> MDVDLFKLSLDDTSSVKGSLLDTRFAQVRVVIPKAMAGGNELLNSNLYDILVVDNNFRAAAALAHTHIIEGQIKCVCTINLPENTGCCLALCVNSSNRGQFSTDIYTIGSQDRMLWNPACSKNSTFTFNPNPCGTGWSLEFLRRTKFHISVVCVSGWSAQPQTDLVMTMDFFVANVPCVPRIYNLGSPGQTLWLNRWMGKLSFGQGVSNDIKSMPLAIGGGAGAKDSILMNMTNAYLSLWRY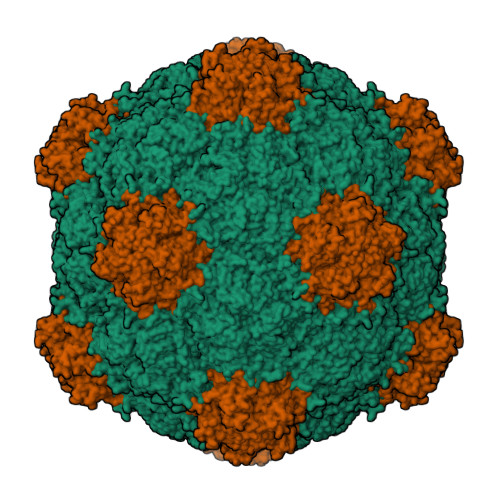FHGDLVFEVNKMSSPYIKSTVTFFIGFGGVSFQPELEDFPNKLVQFSEVQEKIELKFTRAEFLTAWSTQVDPAAQLANDGCPYLYAMVHDSTASTIVGDFNLGVTLTRIENFAGIGCNPGIQGARLLGSAIATPQ;> NAVVRSSPGIYSNCFSLRAPLKPDGPKSFTCDLMGGGVVTDGDTGWQVTVRNTPVSNLLRTAAWKRGTVHVQVVLAGASVKRSDWDSTVQIFLRQSMATSSYDAKIWDICQPGAAMLEFSFDVVGPNSGFEMWDSNWASQTSWFLEFLISNPAQNTLFEVNLRLDENFSVAGTTLMPPFVLDRVSVARPLLGKQTKTVARSARVVRETKEASESP>[4x]MASWSHPQEKGALEVLFQGPMKFSNITIKNFRNFE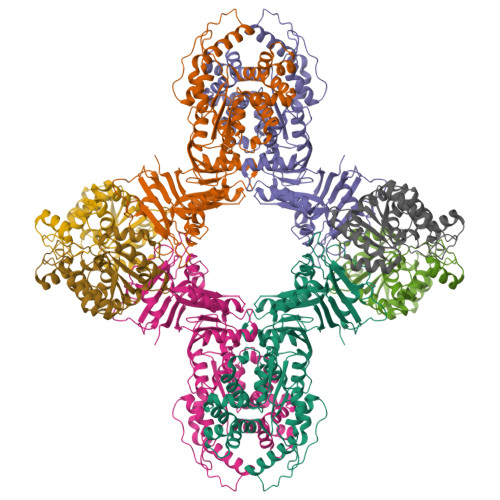KVNINLDNKNVIFGMNDIGKTNFLYALRFLLDKEIRKFGFNKSDYHKHDTSKKIEIILTLDLSNYEKDEDTKKLISVVKGARTSANADVFYIALESKYDDKELYGNIILKWGSELDNLIDIPGRGNINALDNVFKVIYINPLVDLDKLFAQNKKYIFEESQGNESDEGILNNIKSLTDQVNQQIGEMTIIKGFQQEITSEYRSLKKEEVSIELKSEMAIKGFFSDIIPYIKKDGDSNYYPTSGDGRRKMLSYSIYNYLAKKKYEDKIVIYLIEEPEISLHRSMQIALSKQLFEQSTYKYFFLSTHSPELLYEMDNTRLIRVHSTEKVVCSSHMYNVEEAYGSVKKKLNKALSSALFAERVLLIEGPSEKILFEKVLDEVEPEYELNGGFLLEVGGTYFNHYVCTLNDLGITHIIKTDNDLKSKKGKKGVYELLGLNRCLNLLGRENLDEITIDIPEDIKGKKKKERLNERKKEIFKQYKNEVGEFLGERIYLSEIDLENDLYSAIGESMKRIFENEDPVHYLQKSKLFNMVELVNNLSTKDCFDVFEHEKFACLKELVGSDRG;>MSREQIIKDGGNILVTAGAGSGKTTILVSKIEADLKENKTHYSIAAVTFTNKAAKEIEGRLGYSSRGNFIGTNDGFVESEIIRPFIKDAFGNDYPDNFTAEYFDNQFASYDKGLQVLKYQNILGTYSNPKKNFKFQLALDILKKSLVARQYIFSKYFKIFIDEYQDSDKDMHNLFMYLKDQLKIKLFIVGDPKQSIYIWRGAEPENFNGLIENSTDFNKYHLTSNFRCCQDIQNYSNLFNEETRSLIKEKNEVQNVISIADDMPISDILLKLTEEKQVLNIEAELVILVRRRNQAIEIMKELNEEGFNFIFIPQTPLDRATPNATLLKEVIKYVKNDRYSIYDLAAEIVGNLSSREIKEIQKIINELLVPNINQVLINQVLINLFAKLEITLDTREITAFTEVMMTNEFDIAFDTNEYLHKIFTVHSAKGLEFNQVIITASDYNVHYNRDTNEHYVATTRAKDKLIVIMDNKKYSDYIETLMKELKIKNIIKSI[4x]> QRAKVAMSHFEPHEYIRYDLLEKNIDIVRKRLNRPLTLSEKIVYGHLDDPANQEIERGKTYLRLRPDRVAMQDATAQMAMLQFISSGLPKVAVPSTIHCDHLIEAQLGGEKDLRRAKDINQEVYNFLATAGAKYGVGFWRPGSGIIHQIILENYAYPGVLLIGTDSHTPNGGGLGGICIGVGGADAVDVMAGIPWELKCPKVIGVKLTGSLSGWTSPKDVILKVAGILTVKGGTGAIVEYHGPGVDSISCTGMATICNMGAEIGATTSVFPYNHRMKKYLSKTGRADIANLADEFKDHLVPDPGCHYDQVIEINLSELKPHINGPFTPDLAHPVAEVGSVAEKEGWPLDIRVGLIGSCTNSSYEDMGRSAAVAKQALAHGLKCKSQFTITPGSEQIRATIERDGYAQVLRDVGGIVLANACGPCIGQ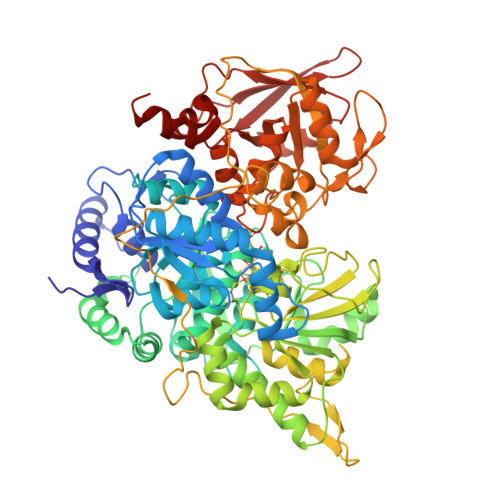WDRKDIKKGEKNTIVTSYNRNFTGRNDANPETHAFVTSPEIVTALAIAGTLKFNPETDFLTGKDGKKFKLEAPDADELPRAEFDPGQDTYQHPPKDSSGQRVDVSPTSQRLQLLEPFDKWDGKDLEDLQILIKVKGKCTTDHISAAGPWLKFRGHLDNISNNLLIGAINIENRKANSVRNAVTQEFGPVPDTARYYKQHGIRWVVIGDENYGEGASREHSALEPRHLGGRAIITKSFARIHETNLKKQGLLPLTFADPADYNKIHPVDKLTIQGLKDFAPGKPLKCIIKHPNGTQETILLNHTFNETQIEWFRAGSALNRMKELQQK> APMGSDPATACCFSYTARKLPR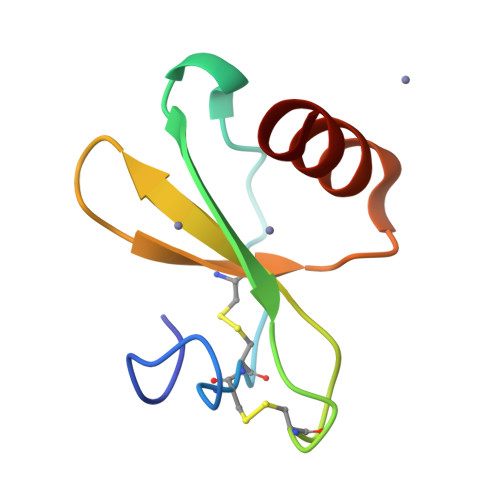NFVVDYYETSSLCSQPAVVFQTKRSKQVCADPSESWVQEYVYDLEL(4S)-3-(4-chlorobenzene-1-carbonyl)-1,3-thiazolidine-4-carboxylic acid | C11 H10 Cl N O3 S | 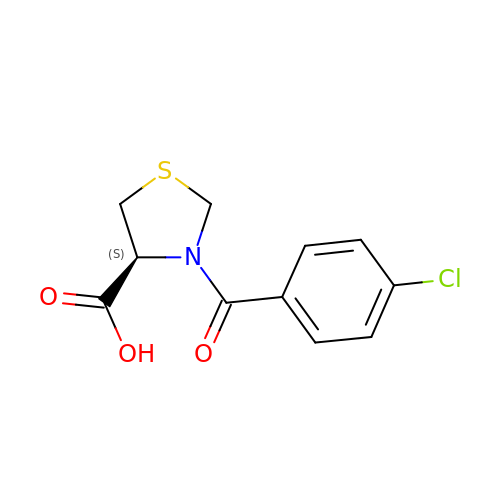SUAAPVQQVPKSHG-SECBINFHSA-N>GSSPEKPTPNGGIPHDNLVLIRMKPDENGRFGFNVKGGYDQKMPVIVSRVAPGTP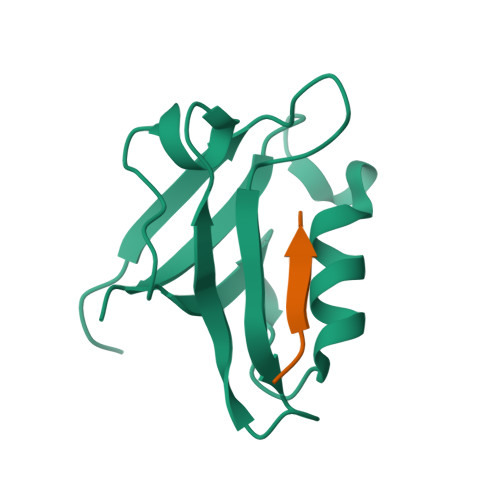ADLCVPRLNEGDQVVLINGRDIAEHTHDQVVLFIKASCERHSGELMLLVRPN[4x];>SWESHKSGRETEV[4x]> ASRYLTDMTLEEMSRDWFMLMPKQKVAGSLCIK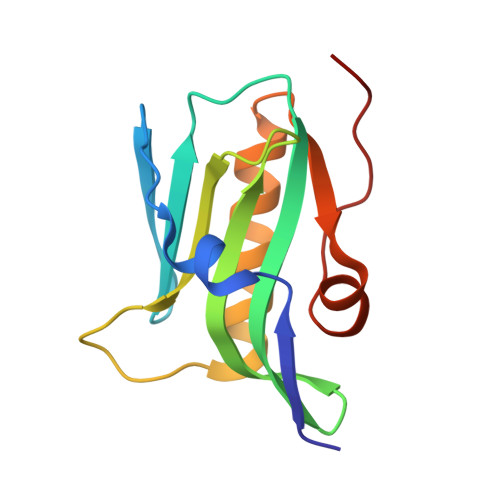MDQAIMDKTIILKANFSVIFDRLETLILLRAFTEEGAIVGEISPLPSLPGHTGEDVKNAIGVLIGGLEANDNTVRVTETIQRFAWRNSDEDGR> EYTGITYISGPLLFVENAKDLAYGAIVDIKDGTGRVRGGQVIEVSEEYAVIQVFEETTGLDLATTSVSLVEDVARLGVSKEMLGRRFNGIGKPIDGLPPITPEKRLPITGLPLNPVARR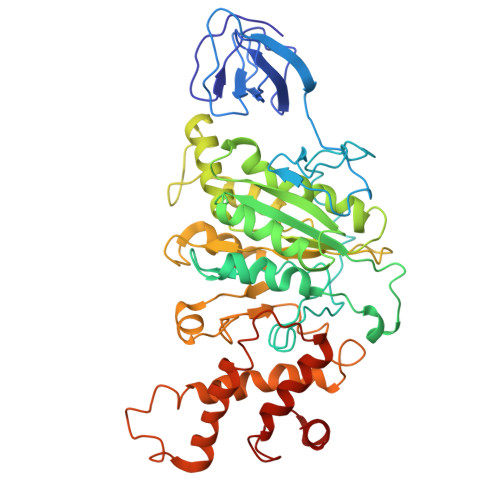KPEQFIQTGISTIDVMNTLVRGQKLPIFSGSGLPANEIAAQIARQATVRPDLSGEGEKEEPFAVVFAAMGITQRELSYFIQEFERTGALSRSVLFLNKADDPTIERILTPRMALTVAEYLAFEHDYHVLVILTDMTNYCEALREIGAAREEIPGRRGYPGYMYTDLATIYERAGVVEGKKGSVTQIPILSMPDDDRTHPIPDLTGYITEGQIQLSRELHRKGIYPPIDPLPSLSRLMNNGVGKGKTREDHKQVSDQLYSAYANGVDIRKLVAIIGEDALTENDRRYLQFADAFERFFINQGQQNRSIEESLQIAWALLSMLPQGELKRISKDHIGKYY> GPLGSMEGAPDINIILENSLSPDATLRHAAEQQLTHAAETNFSQYLLTLVQALANESSEGHIRAAAGIALKNAFSAREFAR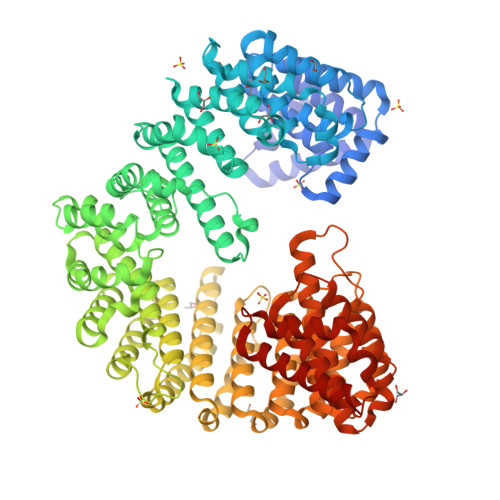QAALQAKWLNQTDQETRTRVKQLALETLASPNSKAGQAAAQVIAAIAAIELPRNQWPELMHALVRNASEGGQHQKQASLTAIGFICETQDTDLRNSLVGHSNAILTAVVQGARKEEPNNEVRFAAITALGDSLEFVGNNFKHEGERNYIMQVVCEATQAQDSRIQQGAFGCLNRIMALYYEHMRYYMEKALFGLTILGMKSDDEDVAKLAVEFWSTVCEEEIAIEDDNAQVESSEQMRPFYNFARVATNEVVPVLLQLLTKQDEDASDDEYNISRAAYQCLQLYAQAVGSTIIPPVIQFVEHNLRHADWHFRDAAVSAFGAIMDGPEEKVLEPIVKTGMQPLIAMMEDESIQVRDSTAYALGRITEACSEAIDPNTHLEPLIRSLFNGLMNSPKMAASCCWALMNIAERFAGEPGAAQNPLTPHFNQSVTNLLTVTAPMNGDSTVRTAAYEVLSVFVQNAANDSLSAVASLSTVILQRLEETLPLQQQVVSVEDKLILEDMQTSLCTVLQATVQRLDKEIAPQGDRIMQVLLQILSTCGGKSSVPEGVFAAISALANAMEEEFAKYMEAFAPFLYNALGNQEEPSLCSMAIGLVSDVTRSLGERSQPYCDNFMNYLLGNLRSTTLANQFKPAILQCFGDIASAIGGHFETYLTIVAQVLQQAATITAGPDGSYEMIDYVISLREGIMDAWGGIIGAMKTSNKTNVLQPYVESIFALLNSIANDPNRSEALMRASMGVIGDLADAYPNGQLADAFRQDWITAMIRETRSNREFGARTIETARWAREQVKRQIAGSQTVMQQS> MDQSVSNVDKMSAFEYNKMIGHGINMGNALEAPVEGSWGVYIEDEYFKIIKERGFDSVRIPIRWSAHISEKYPYEIDKFFLDRVKHVVDVALKNDLVVIINCHHFEELYQAPDKYGPVLVEI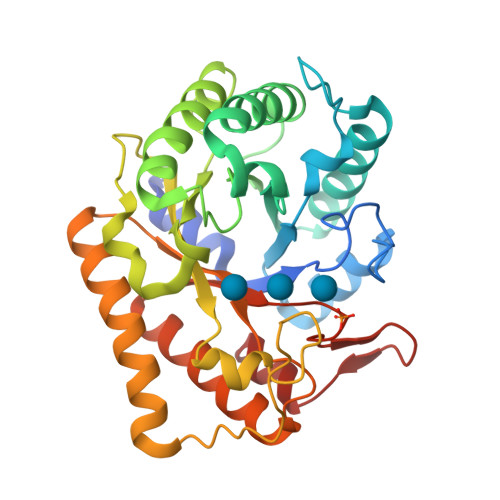WKQVAQAFKDYPDKLFFEIFNEPAQNLTPTKWNELYPKVLGEIRKTNPSRIVIIDVPNWSNYSYVRELKLVDDKNIIVSFHYYEPFNFTHQGAEWVSPTLPIGVKWEGKDWEVEQIRNHFKYVSEWAKKNNVPIFLGEFGAYSKADMESRVKWTKTVRRIAEEFGFSLAYWEFCAGFGLYDRWTKTWIEPLTTSALGK>MSDIITTAFEVRPLTSALGAEIHGVRLEDITDADFAELRRLLLKHLVIFIPDQEGWSAESRIAFGRRFGELEEHAYLPHLDGHPQIQIIDSEQNGKIPIWHTDMTYAPNPPIGSVLQIVDGPAQGGDTMWSNQYLAYEGLSAPLRDLLDGLTAVHSIHIPGLDSQAEHPVVRVHPETGRRALFVNRAHTSHIAQLNRNESDALLQYLYRFSTSPEFTCRYQWRPGSVAIWDNRVTQHYAVDDYSEHR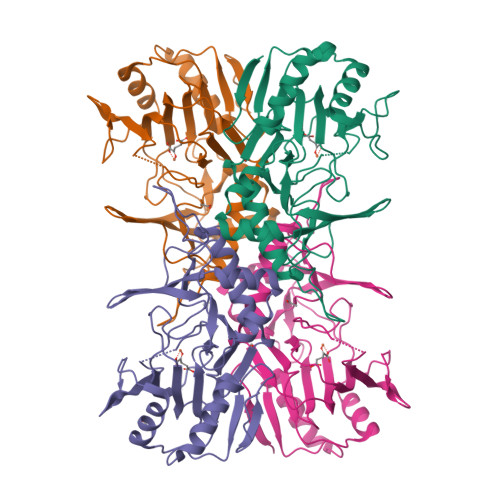RGLRVVVLGDTPSGDKPRWDHYRPVPGQRYVPDWVNAKEAYGKLENLYFQ[4x]>MVMENKTVIPHAKGLKGTIKVPGDKSISHRAVMFGALAKGTTTVEGFLPGADCLSTISCFQKLGVSIEQAEERVTVKGKGWDGLREPSDILDVGNSGTTTRLILGILSTLPFHSVIIGDESIGKRPMKRVTEPLKSMGAQIDGRDHGNLTPLSIRGGQLKGIDFHSPVASAQMKSAILLAGLRAEGKTSVTEPAKTRDHTERMLEAFGVNIEKDGLTVSIEGGQMLTGQHVVVPGDISSAAFFLVAGAMVPHSRITLTNVG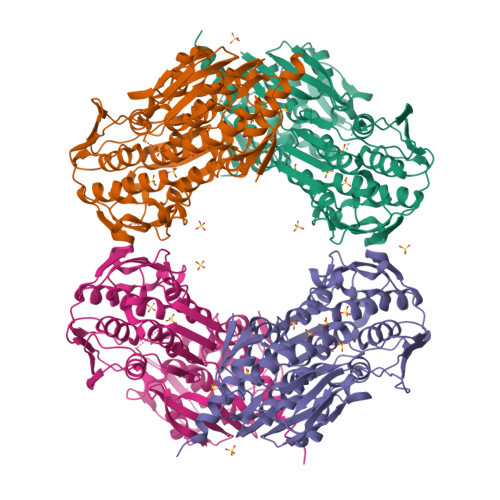INPTRAGILEVLKQMGATLAMENERVQGGEPVADLTIETSVLQGVEIGGDIIPRLIDEIPIIAVLATQASGRTVIKDAEELKVKETNRIDTVVSELTKLGASIHATDDGMIIEGPTPLKGGVTVSSHGDHRIGMAMAIAALLAEKPVTVEGTEAIAVSYPSFFDHLDRLKSEAENLYFQSHHHHHHWSHPQFEK[4x]> MQKDYQKLIVYLCDFLEKEVQKRGF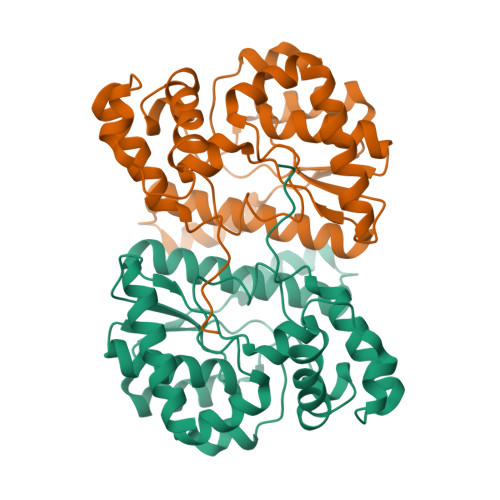KKVVYGLSGGLDSAVVGVLCQKVFKENAHALLMPSSVSMPENKTDALNLCEKFSIPYTEYSIAPYDAIFSSHFKDASLTRKGNFCARLRMAFLYDYSLKSDSLVIGTSNKSERMLGYGTLFGDLACAINPIGELFKTEVYELARRLNIPKKILNKPPSADLFVGQSDEKDLGYPYSVIDPLLKDIEALFQTKPIDTETLAQLGYDEILVKNITSRIQKNAFKLELPAIAKRFNPELEHHHHHH> MENLAKIRMSQKLACWQQILTTLGTSSMSEQEWNT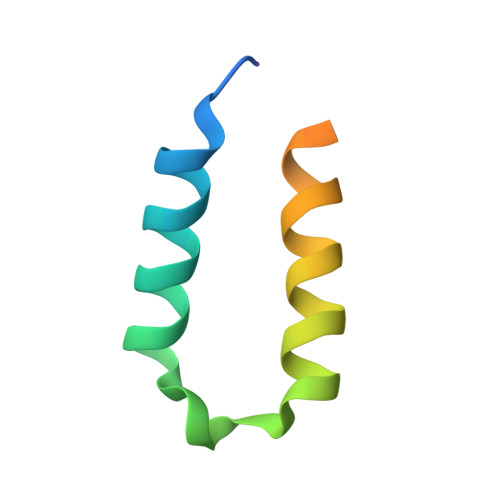FFRGFLESWQNPYCIQTSCDPSIPL> MGSHHHHHHHHHHHHGSPRQLVRRRKKTVMQRYAHFLAHHPFLILTLTFCANIVL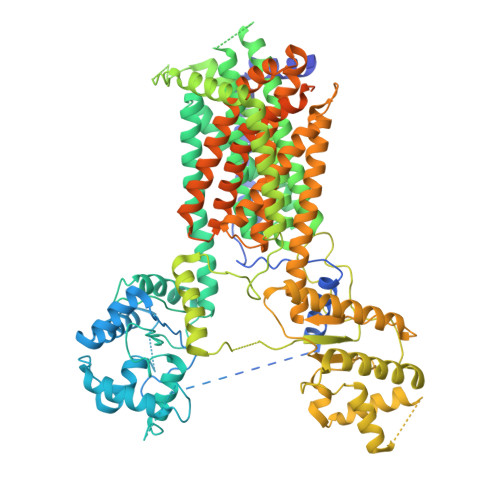LLVIVCTDSLPAFDDPQAGFEPRGSLINQRAQAWRNFLERDGVVQPSTRRKATTTKPVAARQNAPVQEIGTGLRNSTVKENVFSSSGMASLGPITQPRGFFCSRPLLGHAKLILRRKDAGNLLNLEGIRELCQLDADIRRLDEFQSCSEESADTGRLCRTWNLPNYVAVLAGKTSCHQLEEHDIRNVLNLTATCLPFYRSGQLKADCSTSEDDGKTMQEDTITCPGVPTDCIKDSSIYHLLYFISDKESRETGYSSMKHTLAVLPVWSSPAALPLYRALQWGNFTRPDDDGPIQVIGMEMGLGDRLFNTALLEDTLYVGVAAGVVVVVLWLYTGSLFVTLMNLMAIFFSLVVSYFLYVFVFRLTFFPFMNLLTCVIIVAIGADALVIFARLWHLAKTEKDDGRFEKVVHATFRHAAQAILVSSLTASAALFSDIVNPIIAIRCFSIFAGLTVLVHLFFAVTWMPACFVVADKWGSSVYVCTKSPVCRLLYRCRCLHSGLRQYCDYFRIFFEKLLPCLVIRLKWMWMASFVLLTVGACVVVFVFPGLQLASGRTFSLWNSGHPSEQYRLLKDRFAFEENRNLNNNEKVSLHFVWGVLALNQAALLDPTDTGITTMDGRFNMSDPLSQIWMLKFCADLRQQTFFDNSTQSDNACYFDSFMLWMETGACSGHSQFPYPPATFIRCVHTFSNSFPQAKHFGPNFNSLHQIDSFVLRLQTSQLFSHSYTAMQQLHQHVDQWFTAALRTAPPSLQGAWFTGDFAFFDLQQSLISGTALSLIVSLFVAFLVLFFTTLNVGVSLIAITVIAGIMLATTAALVLMEWQLSVFESTIIGLAIGLSVDFTLHYAVSYCCAESYEERELKTNIVISEMASCVTMSAVTTFLAGALMIPSDILFYRQLGLFIITVTAISLLYATIFLPACLAVLGPQGAFLQFHYPSCRPLCCRPDPSKLVEKSMHSSAEFDTTYTTGGTYDHHRETKQCFHQSINQPYQGKALRSPSAAANNHHVVVISATPEQPPKTHPALLLDVDPDLADEETDSVGELGSVPTSRGPSRGTSLIGTLEVLFQ> GSHMTDNLPDRSSVTNNMARVELPVINITSFGTKPSFLNIQKSASTKSLNLIAENSGDTETKEFESSESVVLNHLNRYVFPGSLLMGNSIQDLNYKPVFASLNPITVSLSIPAINQNTAITITNPSLSATRAAVYNYLKTADFTQNGQLSYSIQQFSSYDELKVAFGSNVNSRNLFGKNSSSTNVEEGMVARQSGFYVKFYQTSFTLDMDVPNGSLVKDNNFDSEGIEPVYVSSISYGRMGILAIETNEKAEDAKRIINETFNKLFYKKQTNFSQEEKSFIEGADFNLYLVGGDGSTASQSFKGYEAFVNHVSQGTFSKDQPGVPIFCSYSYLKDNSPVKTKFKFDIKRPPLYVKLVKENMKDINFNDPDGGIYDNKKEAILKIYFYKNRSLVPTLPNPYINFKIREKKKKWQSIAPVYYSSLDQVPFNISERILTKQNTLQNIFATIQTQDNTEFSLISRIIRGGGRQNPVPAGFRAIEINDYELVEDSNYIIIKD

A recently found family of pore-forming toxins, called CDC-like proteins (CDCLs), are wide-spread in gut microbes and are a prevalent means of antibacterial antagonism. Analysis of the CDCLs belonging to the phylum Bacteroidota revealed the presence of sets of two-component CDCLs, one long CDCL (CDCLL) with four domains and one short CDCL (CDCLS) lacking the fourth C-terminal domain, that act as a bicomponent complex via a mechanism only previously observed in the mammalian complement MAC. Unlike CDCs, the CDCLs require proteolytic activation with both components containing a proteolytically cleavable activation loop critical to the regulation of pore formation. Here, we present the crystal structure of a proteolytically activated CDCLL and cryo–electron microscopy (cryo-EM) structures of a prepore-like intermediate and the transmembrane pore.

We determined the crystal structure of act-EaCDCLL to 2.49-Å resolution, revealing the absence of electron density for the D2 β1 strand and its preceeding N-terminal extension, consistent with the MS results above that the peptide dissociates from the protein. Overll, the crystal structures of pro- and act-EaCDCLL superimpose closely, except for differing orientations of domain 4 (D4) with respect to the rest of the domains (33.5° rotation around y axis, shift of 1.4 Å on both x and y axes). We attribute this to altered crystal packing between the two structures and likely flexibility of the domain interface due to very limited interdomain contacts. One notable difference between the pro- and act-EaCDCLL crystal structures is the slight outward movement (1.2 Å) and shortening of the β5 strand (~15 to ~6.5 Å) in the core D3 β sheet in the activated structure. Movement of this strand in CDCs is critical for oligomerization and assembly of the prepore state. The crystal structure of act-EaCDCLL suggests that its activation loop plays a similar role in triggering structural changes that allow for oligomerization, as we observe an initial movement of the β5 strand away from the β4 strand that forms oligomeric interactions in CDCs. Previously, the C11-type protease family was identified as the proteases that activate CDCLs in vivo. This yields the act-EaCDCLL lacking the activation loop and preceding N terminus that also displays movement of the β5 strand away from the CDC-like β4 strand oligomerization interface. Thus, this experiment shows that the D4 of CDCLL is necessary for membrane binding and recruiting CDCLS to form the pore.>[4x]MASPALISDTDQWKALQAHVGAIHKTHLRDLMTDADRCKAMTAEFEGVFLDYSRQQATTETVDKLFKLAEAAKLKEKIDKMFKGEKINTTENRSVLHVALRAPRDAVINSDGVNVVPEVWAVKDKIKQFSETFRSGSWVGATGKPLTNVVSVGIGGSFLGPLFVHTALQTDPEAAESAKGRQLRFLANVDPVDVARSIKDLDPATTLVVVVSKTFTTAETMLNARTIKEWIVSSLGPQAVSKHMIAVSTNLKLVKEFGIDPNNAFAFWDWVGGRYSVCSAVGVLPLSLQYGFPIVQKFLEGASSIDNHFHTSSFEKNIPVLLGLLSVWNVSFLGYPARAILPYSQALEKLAPHIQQLSMESNGKGVSIDGVRLPYEAGEIDFGEPGTNGQHSFYQLIHQGRV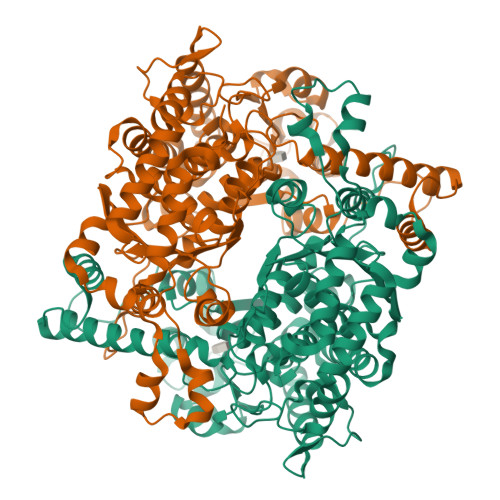IPCDFIGVIKSQQPVYLKGETVSNHDELMSNFFAQPDALAYGKTPEQLHSEKVPENLISHKTFQGNRPSLSFLLSSLSAYEIGQLLSIYEHRIAVQGFIWGINSFDQWGVELGKSLASTVRKQLHASRMEGKPVEGFNPSSASLLTRFLAVKPSTPYDTTVLPKV>[2x]RGSHRILNLVKYDLYSIFKSPLTYLAILVVSSLIATQSILMANSMDNPKHIIVYGSVFAAAKWLLLIIGLMFVVKTITRDFSQGTIQLYMSKVKTRVGYIISKTISIILISILFALIHYVILIVVQASSNGKNLAFSKYVDNLWFFLIFLLFFGLFLFLITLASQKTAMIFSLGVFLVLIVPFIKPFITFIPRYGEKVLDAFDYIPFAYLTDKMISSNFDFSNWQWVISLGSIVIFFILNILYVAKKDI;>[2x]MKLEHITKKYGSNVVLNDIDFDFGDSRIVGLIGKNGVGKTTVMKVMNGNIIKFDGKVDIDNADNIGFLIE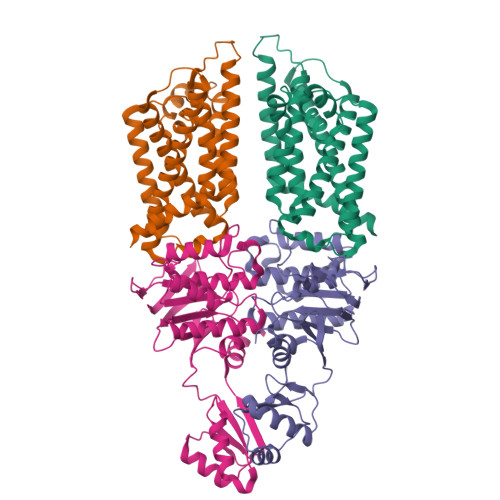HPKLYDNKSGLYNLKLFAQVLGKGFDKAYTDKIIDAFGMRPYIKKKVKKYSMGMKQKLAIAVSLMNKPKFLILDEPTNGMDPDGSIDVLTTIKSLVNELDMRILISSHKLEDIELICDRAVFLRDGHFVQDVNMEEGVASDTTIVTVDHKDFDRTEKYLAEHFQLQNVDKADGHLMINAQKNYQVILKALSELDIYPKYIETRKSSLRDTYFNINQRGDK>MIRNFHSLVKRVPRLALTPFFGFRTSMTLADKKLSTGEASVVLAEKIKGITQQNDITEYGTVISIGDGIARVFGLTKVQAGEMVEFKSGIRGMALNLETDNVGVVVLGNDRDIKEGDVVKRTGAIVDVPIGEAMCGRVFDALGNPIDGLGPLKTTQRARVEIKAPGIIPRQSVRQPMQTGIKCVDSLVPIGRGQRELIIGDRQTGKTAIAIDTILNQKEAFNTGDVKKQLYCIYVAVGQKRSTIANLVSILKQHDCMKFTIVVCATASDAAPLQFLAPYSGCAIGEFFRDNGKHALIIYDDLSKQAVAYRQMSLLLRRPPGREAYPGDVFYLHSRLLERAAKMNDSLGGGSLTALPVIETQAGDVSAYIPTNVISITDGQIFLETELFYKGIRPAINVGLSVSRVGSAAQIKAMKKIAGNLKLTLATYRELAAFSQFGSDLDAKTQQQLNTGERLVEMLKQNQYTPMKVEEQVCIIFAGVKGFLDALVTSEVLKFEKKFLEHVRTNHSALLKRIRDSGDLSEVDTNELNTIIPLFIQEGGFKLKAQ[3x];>MLSKALQRGIARAFSTTAKKEAPKTVKANGQVSQVIGAVVDVQFEGELPQILNALEVQGTQHRLVLEVAQHLGDSRVRTIAMDSTEGLVRGQPVVDTGLPISVPVGPGTLGRIMNVIGEPIDQRGPIKAAKLYPIHRDAPSFTDQATSAEILVTGIKVVDLLAPYARGGKIGLFGGAGVGKTVLIQELINNVAKHHGGYSVFAGVGERTREGNDLYHEMMDSKVISVKEGESRCALIFGQMNEPPGARARVGLTGLTVAEYFRDEEGKDVLLFVDNIFRFTQACSEVSALLGRIPSAVGYQPTLATDLGALQERITTTQKGSITSVQAIYVPADDLTDPAPATTFAHLDATTVLNRGLTELGIYPAVDPLDSTSRMLDPITIGEEHYTVARGVQKLLQDYKSLQDIIAILGVDDLSEEDKLVVARARKVQKFLSQPFFMSEVFSGIPGRFVNLKQNIASFKALLEGAGDEYPESCFYMKGDLEESLA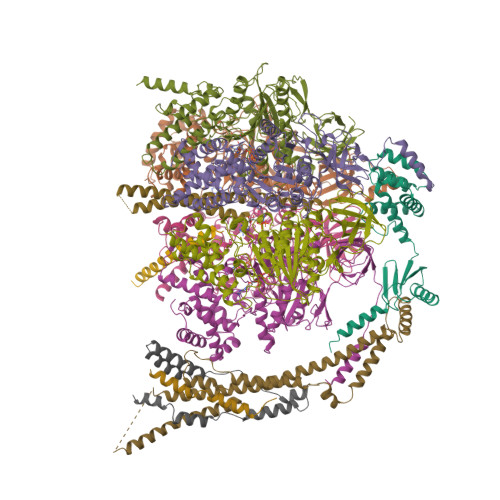AGRADALKSK[3x];> MQVIRKHLAQKGLFNPFLFNRFSTQQDITSVPGDKPPAIEDSIHGKYAGVLFSSASSNKSLNKVAEDMKYFNQLYKESEVFKSFLNNVSLKRNQQRDIISALGKTNFNPATNNLLETLIENKRLDSLPKIAEKYMDYYRILNKQESITIISAQELTAAEKQKVEQGLKKGNANVQFTVVYQVDPAILGGLQMYSGNNFLDCSLLSRVNKLKTEIAKISF;> MHSTLRVFTKNNCLSFTNMNRFSTAAQVAQANYSKFRADYSASVAAFQQRIKTIEKENTGSMKKPMAKAYEHPYNSEHHPLNFSAVKIAETFHDFIGPEQVSPHYESFAMSRKFLLTFWGGFFVLNFGMATVDLNWIMKSTYIPWIFWFQLMYFYVEGKNSMFMPLLQRFYRRAAANEIFTMEAFYHENIENKLRNLMRITKGQLEYWDIHTSYGEIRADSINNFLANEYLRLQSHITSRALNILKQAQAYETMNQAALLQKLIDDATSAIDNALKGDKKAEVLARSLDSAIDGLSKGYMDYQNDPLLPLILSSIEANVKKITTLSAQEQANLIGLTAEQLKSIKENDVRARKEFLESQPKLDNNLKNIESVKKILATWGK;> MSMLAKIAKNVVKTQALKNTTAAQTPSFQAPGNQDKILKWISTLSNKATTGESRSYCTQLSSLVSFYNKQHVEQIPTIDFNEWKSVISTQGLVDKVKENYESLIKEQYNTDAISKQISSASSKALDDIENELSFHAAIWLNAYADYTMFLFELEEYNDPNDYLMHENFDFFRGLETELEELTETHNYIPGAKDDVNLRGYLATQFAWGKKVISFYRHPADDFKCAKATKNMLGR;> MFGLASKGFINTSLVMVPQMNFGANLKQLKIRMKAIGSIKKITKAMKMVAASKMKAETSRLENGRNFAVGSVQKMLENESYVQKKKSTTAPKSTLLVPITSDKGLCGSVNSSIVREVKRLALNNRSAFGLLPVGEKGSSGLSRPFPDLLKSSIVNIQNVNFPTAAAIAHQVSTQGAGYDQVTLIYNHFKNAISYVVKHQELLPRAQFLNLFKYVTRHEAVEPELEYSKNYFFELYMASSVYNALLNSSASEQASRMNAMENASKNAGEILSKLTLDYNKARQAKITMELIEIISGASIV;> MNRSVNIAKNLIQTYRAMSVQSRFAFSTREEEWLDKRTKSQEKVYFDQEDRKAMKRLLEKLNTTSKFVEDSEYLAPQNLEVENILKRYHINYTQALIDELVDWKTGKN;> MNSLSSKKANSLVFKSIRNFTLQWGSLAERPMVDRVMSTSTWPVPYYQRLFKAYPIREKKDKMSLLLSDIDIDDTNWYQAKDFLRGSFRGRQIVDYVENNIASNTYILIQQDVANMAKAYVHDICGYIDVANKENVRILSKGDLI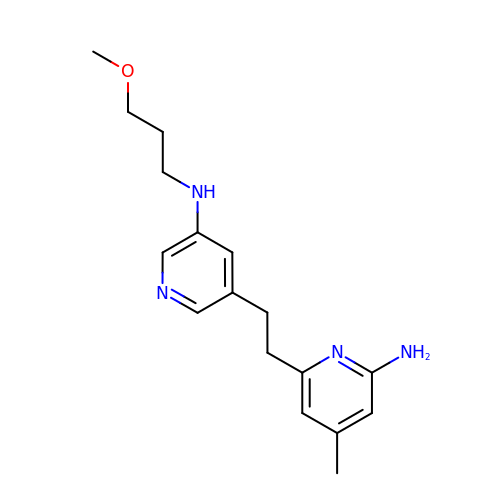6-(2-(5-(3-methoxypropylamino)pyridin-3-yl)ethyl)-4-methylpyridin-2-amine | C17 H24 N4 O | DFYOVMPZILDHIP-UHFFFAOYSA-N>[2x]MKCTIPEQQKVILIDEIGGYDVIKYEDYPVPSISEEELLIKNKYTGVNYIESYFRKGIYPCEKPYVLGREASGTVVAKGKGVTNFEVGDQVAYISNSTFAQYSKISSQGPVMKLPKGTSDEELKLYAAGLLQVLTALSFTNEAYHVKKGDYVLLFAAAGGVGLILNQLLKMKGAHTIAVASTDEKLKIAKEYGAEYLINASKEDILRQVLKFTNGKG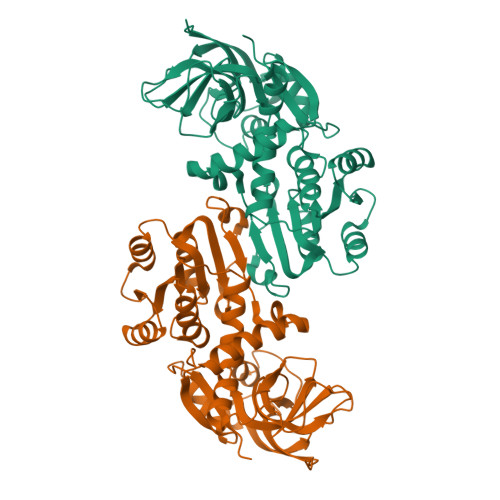VDASFDSVGKDTFEISLAALKRKGVFVSFGNASGLIPPFSITRLSPKNITLVRPQLYGYIADPEEWKYYSDEFFGLVNSKKLNIKIYKTYPLRDYRTAAADIESRKTVGKLVLEIPQ>MGMKALILVGGFGTRLRPLTLSFPKPLVDFANKPMILHQIEALKAVGVDEVVLAINYQPEVMLNFLKDFETKLEIKITCSQETEPLGTAGPLALARDKLLDGSGEPFFVLNSDVISEYPLKEMLEFHKSHGGEASIMVTKVDEPSKYGVVVMEESTGRVEKFVEKPKLYVGNKINAGIYLLNPSVLDKIELRPTSIEKETFPKIAAAQGLYAMVLPGFWMDIGQPRDYITGLRLYLDSLRKKSPAKLTSGPHIVGNVLVDETATIGEGCLIGPDVAIGPGCIVESGVRLSRCTVMRGVRIKKHACISSSIIGWHSTVGQWARIENMTILGEDVHVSDEIYSNGGVVLPHKEIKSNILKPEIVMKLAAALEHHHHHH[4x]

Plant vitamin C biosynthetic pathway contains conversion of D-mannose-1-phosphate (Man-1-P) to GDP-D-mannose (GDP-Man), a step catalyzed by the Man-1-P guanylyltransferase which is commonly named GDP-Man pyrophosphorylase (GMPase). Arabidopsis thaliana VTC1 is the first genetically characterized plant GMPase and has unique properties when compared with bacterial and animal homologs. Structures of two GMPases have been reported, which are the crystal structure of GMPase from the hyperthermophilic bacterium Thermotoga maritima (TmGMP) and the cryo-EM structure of human GMPase (GMPPA-GMPPB complex) that is arranged into a dodecamer. These structures show that an oligomer-forming monomer (protomer) of GMPase consists of two domains: an N-terminal Rossmann fold-like domain and a C-terminal left-handed β-helix (LβH) domain. VTC1 dimerizes via its LβH domain and forms a dodecamer in crystal.

The 3.0-Å product-bound structure was solved based on the unliganded VTC1 structure. Different from the unliganded structure, the overall structure of product-bound VTC1 has a threefold symmetry with each asymmetric unit having two dimers. Six dimers form a dodecameric assembly in shape of a three-petaled flower. The two dimers within an asymmetric unit bind a total of one GDP-Man, two inorganic PPi, and two citrates. Specifically, the stalk protomer binds a citrate, the middle protomer binds a GDP-Man and a citrate, and the inner and outer protomers each bind a PPi. The two dimers can be aligned with a root mean square deviation of 0.49 Å. Their superimposition demonstrates that citrate and PPi bind to the same site on catalytic domain. The product GDP-Man binds at the edge of the central β-sheet. The oxygen at guanine C6 forms a hydrogen bond with the backbone amide of Gly85, the guanine N1 forms two hydrogen bonds with the side chain of Asp80, and the hydroxyl groups at C2 and C3 of D-mannose form hydrogen bonds with the side chain amide of Asn173 and the backbone amide of Gly146, respectively. The pyrophosphate moiety of GDP-Man is flanked by, but not directly interacting with the catalytically critical residues Glu195-Lys196, Asp111, and Asp219. It makes direct polar contacts with the backbone amide groups of Gly9, Thr12, and Arg13, the hydroxyl group of Thr12, and the guanidino group of Arg13. PPi binds to the same site as citrate, but in the inner protomer, the interacting residues differ from the afore-mentioned residues in that Gly9 is not directly involved and Lys23 replaces Arg13 for ligand recognition.> MEKSFVITDPRLPDNPIIFASDGFLELTEYSREEILGRNGRFLQGPETDQATVQKIRDAIRDQREITVQLINYTKSGKKFXNLL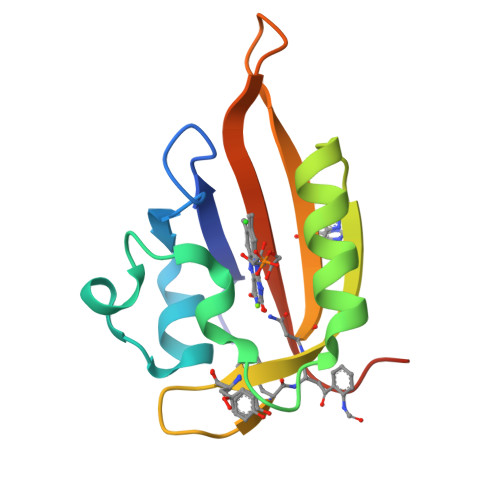HLQPMRDQKGELQYFIGVQLDGEFIPNPLLG EQUILENIN | C18 H18 O2 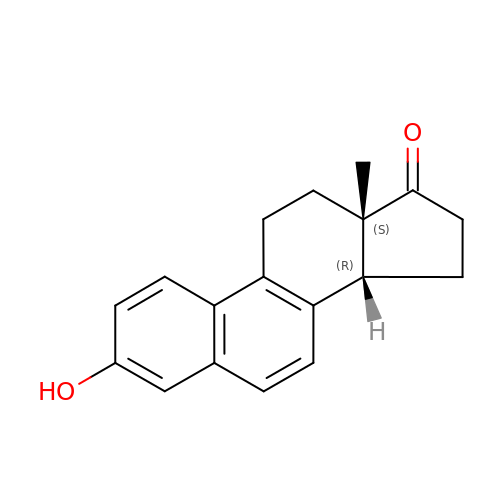| PDRGHUMCVRDZLQ-WMZOPIPTSA-N>[2x]AGKKVLIVYAHQEPKSFNGSLKNVAVDELSRQ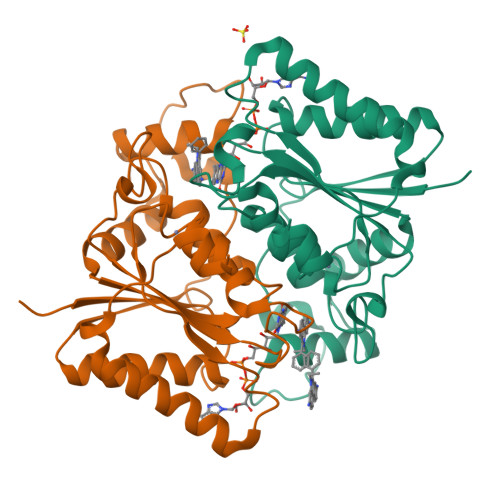GCTVTVSDLYAMNFEPRATDKDITGTLSNPEVFNYGVETHEAYKQRSLASDITDEQKKVREADLVIFQFPLYWFSVPAILKGWMDRVLCQGFAFDIPGFYDSGLLQGKLALLSVTTGGTAEMYTKTGVNGDSRYFLWPLQHGTLHFCGFKVLAPQISFAPEIASEEERKGMVAAWSQRLQTIWKEEPIPCTAHWHFGQ> SNAVMSGNKGTNYEKLYLGMDFGTSGGRFTVIDEQGEIKAQGKREYPPFMKEESMGWASSWKATLFSLLEDIPVTVRSLVSSISLDGTSATTLILNSESGEVLCQPYLYNQSCPDALPEVKSIAPANHTVCSGTSTLCKLVSWWNTEVPNRESAVLLHQADWLLWLLHGRLGVSDYNNALKVGYDPESESYPSWLLGQPYSQLLPKVQAPGTSIGNLKESFTRQFGFPDDCIVCTGTTDSIAAFLAARATEPGKAVTSLGSTLAIKLLSTKRVDDARYGVYSHRLDDKWLVGGASNTGGAILRQLFSDEQLERLSQEINPMVGSPLDYYPLQSSGERFPIADPNLAPRLLPRPESDVEFLHGILESIARIEGKGYKLLKELGATEAEEVLTAGGGAKNDKWIKIRQRVLGLPVKKAVHTEASYGASLLALKGAKQNSGL

Synpcc7942_2462 from the cyanobacteria Synechococcus elongatus PCC 7942 encodes a putative sugar kinase (SePSK), and this kinase contains 426 amino acids. The At2g21370 gene product from Arabidopsis thaliana, xylulose kinase-1 (AtXK-1), whose mature form contains 436 amino acids, is located in the chloroplast (ChloroP 1.1 Server). SePSK and AtXK-1 display a sequence identity of 44.9%, and belong to the ribulokinase-like carbohydrate kinases, a sub-family of FGGY family carbohydrate kinases. Domain I exhibits a ribonuclease H-like folding pattern, and is responsible for the substrate binding, while domain II possesses an actin-like ATPase domain that binds cofactor ATP.

Apo-AtXK-1 exhibits a folding pattern similar to that of SePSK in line with their high sequence identity. However, superposition of structures of AtXK-1 and SePSK shows some differences, especially at the loop regions. A considerable difference is found in the loop3 linking β3 and α4, which is stretched out in the AtXK-1 structure, while in the SePSK structure, it is bent back towards the inner part. The corresponding residues between these two structures (SePSK-Lys35 and AtXK-1-Lys48) have a distance of 15.4 Å. In contrary, limited increasing of ATP hydrolysis activity was detected for AtXK-1 upon addition of D-ribulose, despite its structural similarity with SePSK. Structural comparison of SePSK and AtXK-1 showed that while the RBL1 binding pocket is conserved, the RBL2 pocket is disrupted in AtXK-1 structure, despite the fact that the residues interacting with RBL2 are highly conserved between the two proteins. In the RBL-SePSK structure, a 2.6 Å hydrogen bond is present between RBL2 and Ser12, while in the AtXK-1 structure this hydrogen bond with the corresponding residue (Ser22) is broken. This break is probably induced by the conformational change of the two β-sheets (β1 and β2), with the result that the linking loop (loop 1) is located further away from the RBL2 binding site.>[2x]HQLQPRRVSFRGEASETLQSPGYDPSRPESFFQQSFQRLSRLGHGSYGEVFKVRSKEDGRLYAVKRSMSPFRGPKDRARKLAEVGSHEKVGQHPCCVRLEQAWEEGGILYLQTELCGPSLQQHCEAWGASLPEAQVWGYLRDTLLALAHLHSQGLVHLDVKPANIFLGPRGRCKLGDFGLLVELGTAGAGEVQEGDPRYMAPELLQGSYGTAADVFSLGLTILEVACN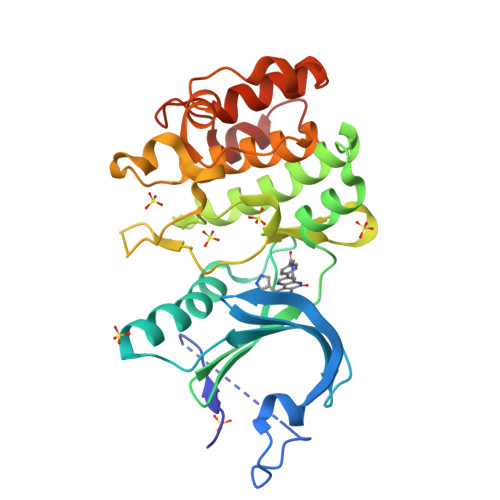MELPHGGEGWQQLRQGYLPPEFTAGLSSELRSVLVMMLEPDPKLRATAEALLALPVLRQP> MASMTGGQQMGVDFVPVESMETTMRS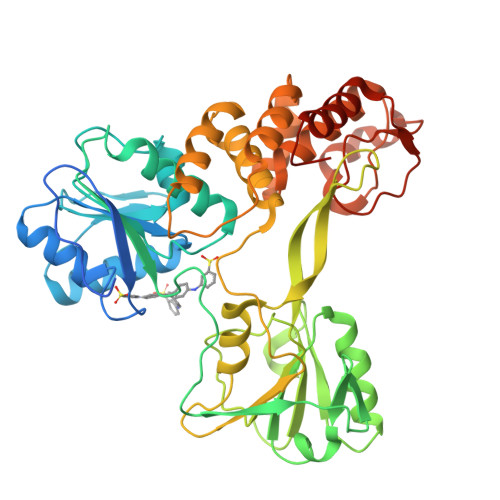PVFTDNSSPPAVPQAFQVAHLHAPTGSGKSTKVPAAYAAQGYKVLVLNPSVAATLGFGAYMSKAHGVDPNIRTGVRTITTGAPITYSTYGKFLADGGCSGGAYDIIMCDECHSTDSTTILGIGTVLDQAETAGARLVVLATATPPGSVTVPHPNIEEIALSNTGEIPFYGKAIPIETIKGGRHLIFCHSKKKCDELAAKLSALGIHAVAYYRGLDVSVIPASGNVVVVATDALMTGFTGDFDSVIDCNTCVTQTVDFSLDPTFTIETTTMPQDAVSRSQRRGRTSRGRRGIYRFVTPGERPSGMFDSSVLCECYDAGCAWYELTPAETSVRLRAYLNTPGLPVCQDHLEFWESVFTGLTHIDAHFLSQTKQAGDNFPYLVAYQATVCARAQAPPPSWDQMWKCLTRLKPTLHGPTPLLYRLGAVQNEVTLTHPITKYIMACMSADLEVVTHHHHHH>PMISEEREPLADVIEKGDEIKVVAEVPGVNKEDIKVKVTNGGKKLVITAKSEDRQYYKEIDLPAEVDEKAAKANFKNGVLEI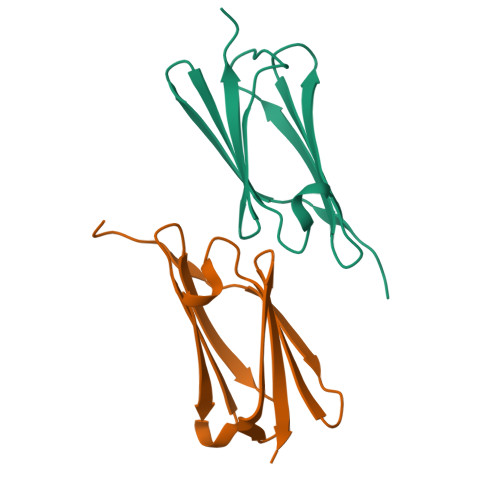TLKKKASS[2x]> MGSPDPKFNGIEEVPEDEIFVEAGVNASGNNFIEIKAIVNNKSGWPARVCENLSFRYFINIEEIVNAGKSASDLQVSSSYNQGAKLSDVKHYKDNIYYVEVDLSGTKIYPGGQSAYKKEVQFRISAPEGTVFNPENDYSYQGLSAGTVVKSEYIP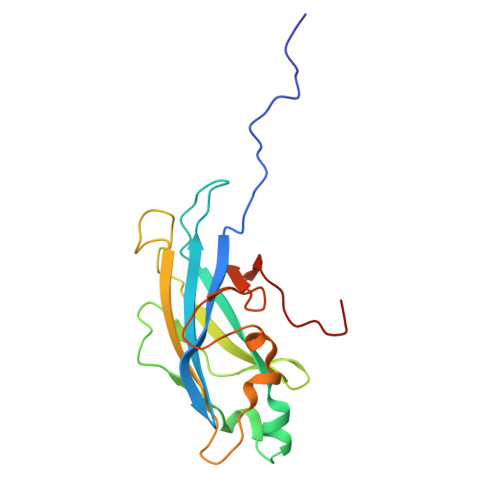VYDAGVLVFGREPLEHHHHHH> MQLNNRDLKSIIDNEALAYAMYTVENRAIPNMIDGFKPVQRFVIARALDLARGNKDKFHKLASIAGGVADLGYHHGENSAQDAGALMANTWNNNFPLLDGQGNFGSRTVQKAAASRYIFARVSKNFYNVYKDTEYAPVHQDKEHIPPAFYLPIIPTVLLNGVSGIATGYATYILPHSVSSVKKAVLQALQGKKVTKPKVEFPEFRGEVVEIDGQYEIRGTYKFTSRTQMHITEIPYKYDRETYVSKILDPLENKGFITWDDACGEHGFGFKVKFRKEYSLSDNEEERHAKIMKDFGLIERRSQNITVINEKGKLQVYDNVVDLIKDFVEVRKTYVQKRI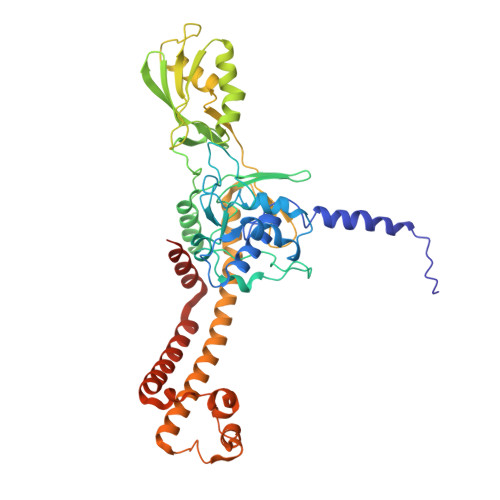DNKIKETESAFRLAFAKAHFIKKVISGEIVVQGKTRKELTEELSKIDMYSSYVDKLVGMNIFHMTSDEAKKLAEEAKAKKEENEYWKTTDVVTEYTKDLEEIKHHHHHHHHHH While reducing NAD(P)+ to NAD(P)H, MEs catalyze the oxidative decarboxylation of the TCA cycle intermediate L-malate to produce the TCA carbon source pyruvate and a byproduct carbon dioxide (CO2) in the presence of divalent metal ions such as a magnesium (Mg2+) ion. The hybrid-type MEs consist of an N-terminal catalytic domain (ME domain) and a C-terminal activity regulating domain. The PTA domain does not possess an enzymatic activity of PTA but acts as an allosteric modulator of catalysis; that is, binding of some metabolites to the PTA domain increases or decreases the enzymatic activity. Binding of acetyl-CoA to the PTA domain is known to reduce the catalytic activity of several hybrid-type MEs.

To find the acetyl-CoA binding site of EcMaeB, we collected cryo-EM data of EcMaeBholo in the presence of acetyl-CoA (EcMaeBacetyl-CoA) and determined its structure at 2.03 Å resolution. The cryo-EM map of the ME domain was ambiguous as is in the cryo-EM data of EcMaeBholo despite the higher resolution. As with EcMaeBholo, local refinement of the ME domain dimer sharpened the NADP+ and Mg ion maps. Due to the ambiguity of the cryo-EM map of the ME domain, detailed discussion on the ME domain structure at an each-residue level is difficult. However, cryo-EM maps for secondary structures show that the ME domain of EcMaeB moves when acetyl-CoA binds to the PTA domain. The movement of the ME domain resulted in a slightly narrower space above the substrate binding site in EcMaeBacetyl-CoA. This observation suggests the possibility that acetyl-CoA binding makes it difficult for the substrate and/or cofactors to bind to EcMaeB.

>[2x]DDQLKQSALDFHEFPVPGKIQVSPTKPLATQRDLALAYSPGVAAPCLEIEKDPLKAYKYTARGNLVAVISNGTAVLGLGNIGALAGKPVMEGKGVLFKKFAGIDVFDIEVDELDPDKFIEVVAALEPTFGGINLEDIKAPECFYIEQKLRERMNIPVFHDDQHGTAIISTAAILNGLRVVEKNISDVRMVVSGAGAAAIACMNLLVALGLQKHNIVVCDSKGVIYQGREPNMAETKAAYAVVDDGKRTLDDVIEGADIFLGCSGPKVLTQEMVKKMARAPMILALANPEPEILPPLAKEVRPDAIICTGRSDYPNQVNNVLCFPFIFRGALDVGATAINEEMKLAAVRAIAELAHAEQSEVVASAYGDQDLSFGPEYIIPKPFDPRLIVKIAPAVAKAAMESGVATRPIADFDVYIDKLTEFVYKTNLFMKPIFSQARK> SENRIAKKML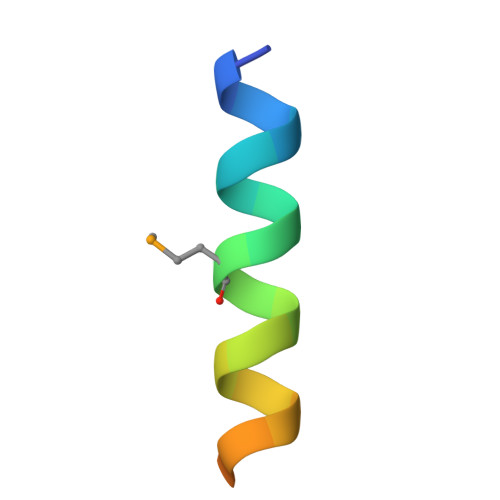LEEIKANLSSDED>TIPDAMIVIDGHGIIQLFSTAAERLFGWSELEAIGQNVNILMPEPDRSRHDSYISRYRTTSDPHIIGIGRIVTGKRRDGTTFPMHLSIGEMQSGGEPYFTGFVR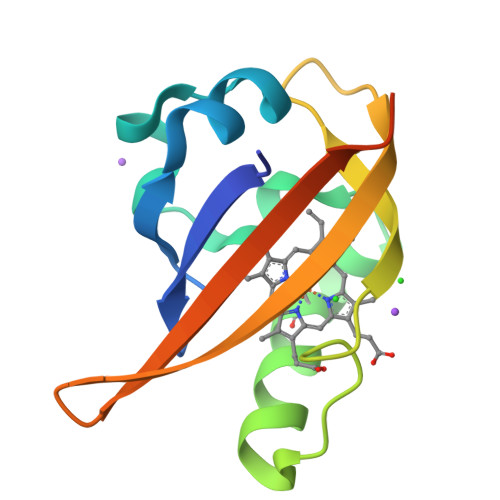DLTEHQQTQARLQEL[2x]>[4x]APACPQFDDRTKAAADRGV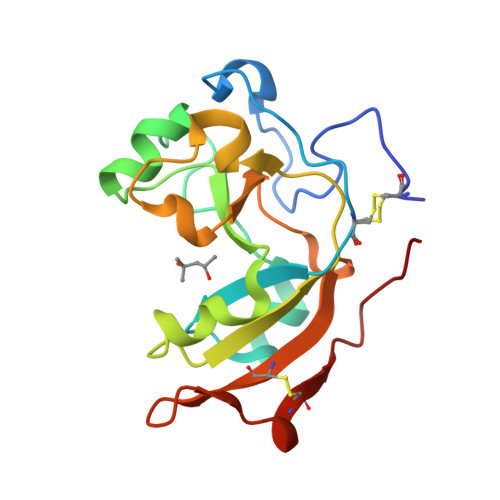DVDRITPEPVWRTTCGTLYRSDSRGPQVVFEEGFHAKDVQNGQYDVEKYVLVNQPSPYVSTSYDHDLYKTWYKSGYNYYVDAPGGIDVNKTIGDTHKWADQVEVAFPGGIQRKYIIGVCPVDRQTKTEIMSDCESNPHYQPWH>[4x]ARTVVLITGCSSGIGLHLAVRLASDPSQSFKVYATLRDLKTQGRLWEAARALACPPGSLETLQLDVRDSKSVAAARERVTEGRVDVLVCNAGLGLLGPLEALGEDAVASVLDVNVVGTVRMLQAFLPDM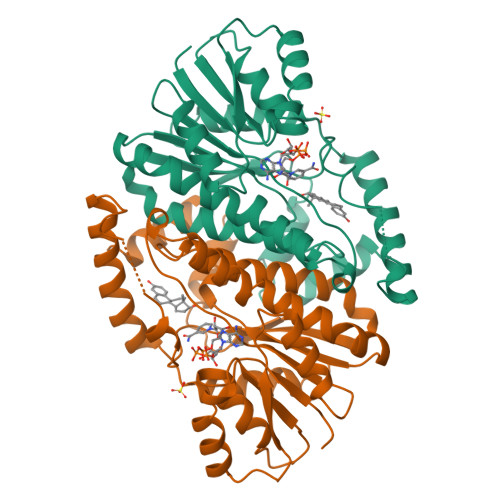KRRGSGRVLVTGSVGGLMGLPFNDVYCASKFALEGLCESLAVLLLPFGVHLSLIECGPVHTAFMEKVLGSPEEVLDRTDIHTFHRFYQYLALSKQVFREAAQNPEEVAEVFLTALRAPKPTLRYFTTERFLPLLRMRLDDPSGSNYVTAMHREVFGDVPAKAEAGAEAGGGRGPGAEDEAGRSAVGDPELGDPPAAPQ> GRATKSIP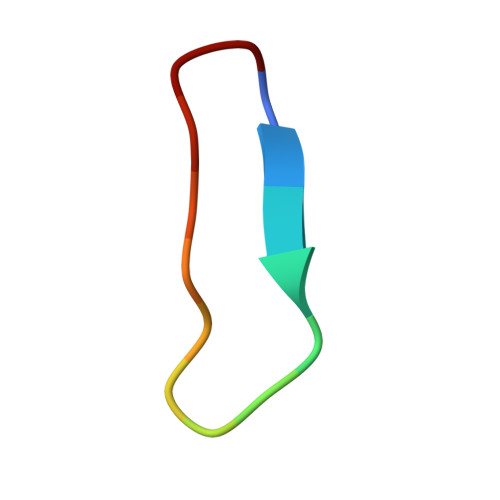PIAFPD> SQPIFLNVLEAIEPGVVCAGHDNNQPDSFAALLSSLNELGERQLVHVVKWAKALPGFRNLHVDDQMAVIQYSWMGLMVFAMGWRSFTNVNSRMLYFAPDLVFNEYRMHKSRMYSQCVRMRHLSQEFGWLQITPQEFLCMKALLLFSIIPVDGLKNQKFFDELRMNYIKELDRIIACKRKNPTSC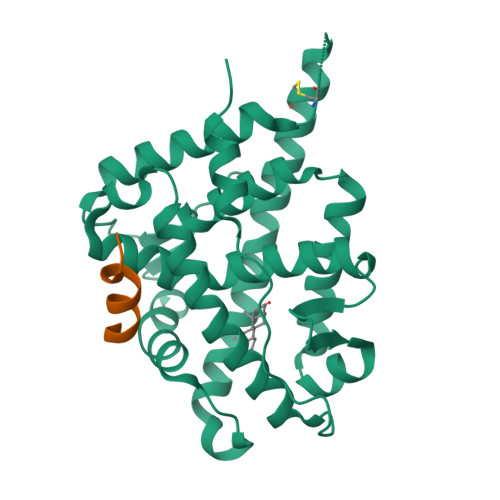SRRFYQLTKLLDSVQPIARELHQFTFDLLIKSHMVSVDFPEMMAEIISVQVPKILSGKVKPIYFHT;> NALLRYLLDRDD> LESKIFRKRWVLLPDYVPDVLPHREAELRRLAEVLAPALRGEKPSNALLYGLTGTGKTAVARLVLRRLEARASSLGVLVKPIYVNARHRETPYRVASAIAEAVGVRVPFTGLSVGEVYERLVKRLSRLRGIYIIVLDEIDFL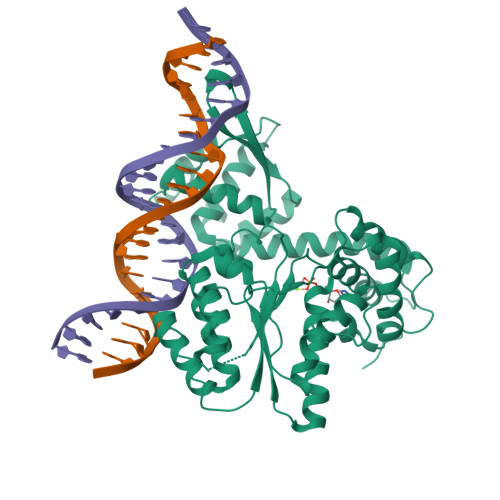PKRPGGQDLLYRITRINQELGDRVWVSLVGITNSLGFVENLEPRVKSSLGEVELVFPPYTAPQLRDILETRAEEAFNPGVLDPDVVPLCAALAAREHGDARRALDLLRVAGEIAERRREERVRREHVYSARAEIERDRVSEVVRTLPLHAKLVLLSIMMLEDGGRPASTGEIYERYKELTSTLGLEHVTLRRVSGIISELDMLGIVKSRVVSRGRYGKTREVSLDADRLAVENALSEDPFVARLL The icosahedron-shaped NCLDVs have a roughly icosahedral outer capsid composed of hundreds of pseudo-hexameric capsomers in the icosahedral faces and one pentameric capsomer at each fivefold vertex. Each pentameric and pseudo-hexameric capsomer is composed of five copies of a penton protein and three copies of a major capsid protein (MCP), respectively. Immediately internal to the outer capsid shell is a layer of minor capsid proteins that stabilizes the outer capsid. PBCV-1 has an outer capsid with a diameter of ~190 nm, an inner bilayer lipid membrane that encloses a 331-kbp genome, and a minor capsid shell in-between the outer capsid shell and the inner membrane.

Here we have extended the fivefold averaged structure of PBCV-1 capsid to near-atomic resolution (~3.8 Å) and obtained an atomic model of the viral capsid by employing a symmetry relaxation procedure to distinguish the unique vertex with the other capsid vertices of PBCV-1, and the “block-based” reconstruction method. The atomic model contains 7135 polypeptide chains from 30 different kinds of proteins, with 15 kinds of the proteins previously unresolved. These previously unresolved proteins include five variants of the MCP that are involved in composing five types of pseudo-hexameric capsomers, one kind of penton protein variant that composes one type of pentameric capsomer, and nine kinds of minor capsid proteins. Type I, type II, type III and type IV capsomers are homotrimers of the MCP, MCPv1, MCPv3 and MCPv5, respectively, while type V and type VI capsomers are heterotrimers, with type V capsomer composed of two MCPv1 and one MCPv2 subunits, and type VI capsomer composed of two MCPv3 and one MCPv4 subunits. Type I capsomers are present in all the icosahedral asymmetric units, while type II and type V capsomers are only present in the unique vertex, with type II capsomers located at position a, b and type V capsomer located at position d, respectively. Each pentameric capsomer in the eleven common vertices of the viral capsid (hereafter “type I pentameric capsomer”) is composed of five penton protein (P1) monomers, whereas the pentameric capsomer in the unique vertex (hereafter “type II pentameric capsomer”) is composed of five monomers of the penton protein variant (P1v1). Compared with the type I pentameric capsomer, the type II pentameric capsomer has an ~7-nm-high “crown” structure formed by the DE insertion of its five P1v1 subunits. However, the association between the type II pentameric capsomer and its neighboring capsomers is reinforced by loop 179–197 of insertion domain I and the C-terminal bridging helix of P1v1. Below the type II pentameric capsomer is a lipid vesicle that has an ~7.3 × 104-Å3-large lumen, which is supported by minor capsid proteins P9, P15, P16, P17, and P18.

>[72x]MAGGLSQLVAYGAQDVYLTGNPQITFFKTVYRRYTNFAIESIQQTINGSVGFGNKVSTQISRNGDLITDIVVEFVLTKGGNGGTTYYPAEELLQDVELEIGGQRIDKHYNDWFRTYDALFRMNDDRYNYRRMTDWVNNELVGAQKRFYVPLIFFFNQTPGLALPLIALQYHEVKLYFTLASQVQGVNYNGSSAIAGAAQPTMSVWVDYIFLDTQERTRFAQLPHEYLIEQLQFTGSETATPSATTQASQNIRLNFNHPTKYLAWNFNNPTNYGQYTALANIPGACSGAGTAAATVTTPDYGNTGTYNEQLAVLDSAKIQLNGQDRFATRKGSYFNKVQPYQSIGGVTPAGVYLYSFALKPAGRQPSGTCNFSRIDNATLSLTYKTCSIDATSPAAVLGNTETVTANTATLLTALNIYAKNYNVLRIMSGMGGLAYAN;>MPGAISQLVSYGAQDVYLTGNPQITFFKAVYRRYTNFAMESIQQTFDGTTDFGKFPTVTISRNGDLAGPIWIEVNLPSLLGYNITPTPAEGNTSNIAAISTVFKDDYNNYWWTYNPGTTPQYSNLIAAFSNVDYKYYANAVTSTYPPTALSNVVYSWPYMITGNTGTRSTVAIPTANLRYVNGIGLALFNSIELELGGQRIDKHYSEWWDIWTELTETAEKIQGYNTMVGRYDPAVYNAGWNISQAQGGTYYVPLKFCYNRNPGLYMPLVALSYHQMKLNFNINNYLNCVKCNYPVTALTSKNGANPLSITNMKLYTDFVFLDAPERIRMSEIQHEYLVTQLQWQGSEPVTAPGDPNGSTNRKITLNFNHPVRELVFVYQAASNYDVDAVTGNNIFDYEIPANPTATPPYAGGGEVFTEVKLIINGSDRFSGRPGAYFRLVQPYEHHVRVPSKSVYVYSFALEDADSRQPNGSANFTRYDSVQLQLTLNENLASGRVQIYAPNFNILRIAAGMGGLAFAN[8x];> MDPTTRFRGSDVPVHNEDHMVFAKPSEIGLQGRQGFYTNTNVVTNTYNHVYTPPGGHTGGKFTQDIYTTDLLIAAKDEKADKIPLDKRMDGTFSEGTFVQLLSRGPQDVYLTYNPQISLFKRKYKRYTNFAIENFEERFSTVVKFGTRNICQLSKNGDLIGNMCFRVTLPNLGIPGGTWAPTMGYNIFSTIRMRIGDTIVQSHDRVWYDIDDKMFCDSTKIQGLDELIKRNVTLTTDQEWELIIPLKFFCCKRNTGKQQFLPILNMDTNINVYLEFNLLPLNSLVTLPTGSILPDIQSIDASVWVDYIFLDDTEKFRFAQDPCVYLIEQTASMDSLSYATTTSGQTYNKTDVYVDMKELNKPVKYVEIIAYEQGSTSFDYVDIIESATFYLNSDEQFKTRAGEYFSLVQPYQHFKRSDPTSNISTFSFALDAGSFQPNGYLNFAPYVRTRFAFKIQPQTTPHVIRLFAVCLNWVKFESGLVKLLFN;>MSGALNQLVAVGKQDAFITGDNLDNSVWRNVTKKVSNFAMESIENYINVNPGSTTSIVVGRFGDLVRKVTLEITMKKGSTTNPFYPSEQYVKYAHLSIGGQIVYRIDDFPTWTRVHEELFMDPDTRATNQRVNNFRPEDPVGAIRKFYLDIPLFFTDDASKALPLIALQYHEVKLDVLFASPGDIPGIDASYTPTVECYIDYVFLDTPEREWFARNTHMYVIEQLQHYNNVFSVAAVEQTKRLNLPFTMPTRYLIWLLKTGADGVYTTSGYPFENNDSYAAIKSAKLQFNGTDRFSERPGYYFTTVQPQDAFGRSPSAGIYVYSFGLDVTGMTSKGALNFSRMDNATLSITTKAATAATISDVYNQSTTLASAITDFTSIAIYAKSFNVLKIDYGMGGMLFAN[11x];>[4x]MVSGGVVQLISYGAQDVYISGGPKTIFKSYVKKVNNFAIDSVKIPINGMGNGNPSVLIPRNGDLIKSIRLEITLKKGTGQSFYPAEQLISYLALKIGGNIIQKIDDFSNFCRIRNELFMDPDERHTDYRVNNFSSSDVVGSVKYFFLDLPLFFSKDTSVALPLIALQYHDIELDFRFNDVSTIQGVDASYTPTIEMYIDYVYLEQQERIKLVEKPLFYNIEQCNFYRKDITFPALSSTFKLDIPFNNPSRFLVWYFNTDSFGIYNTSGLYFNSNDAAAPLESAVMLLNGTERFKSREGMYFNCVQPQQALGRSPSSGIYMYAFGEDVANATSKGALDMSRVNELSLQLTTKNATAANVYTVYNPQETLASSTSTYKGITLFSTNWNVLQVRSGLGAVMFDS;> MDDIETIEKYGRDETYIFLADSAKRDTAAYPTAAEYEVLFNAQFRNVTKFELLEVNIPRTEYLIDSSENTFAYALNQPTNINTWQQEIEGNIRIATITPGDYNLPQLIDEMNNVLQQTANTYGDSVILQVSPVTNPSEISNKIRITASGPFTLLGSTGTIGNTIGFGDPVNTSVASTTGYYSTVPGYSVNYPNGADYVFLSNQGNIGSEAVNEFVGPLPPGDNVSFTPIYTGQTPSQYFIAPSAGVPTTVSAYFVDQATAPPGGFVVNYSIIKVSDSSTIATGSLISTNDDLVPSVSSPSVVSANFIQGQQYYIQFTPGSSGSSAGNCTALWYSFPNLPPVSGAYAAINGTLVFPGQYFCTDVSAGAYGNELTSPGIVNITGARYIKIRCKELEQLIYRDRVGEPTTAGIGIVNLIGYGFERSRYDFSSIPVKAFHPIGKLQKLTFRLERPNGTLYDTNGVDNTMLCALTFKVVPNNAVDKTFDGPGKYPAAPGYSGDYIQLQQKRWGEEARATYPTHKSTYNRCRPRTT;> MCNTYYKRVKFNLFLYTNSIEMELLAVASIIGYGLFSSQQGRETRPDRNRYAEALGSGQGLDEDYDVKPTDMVRKYRKKAEKRWKKAQVPKESGIITPNMRPSEVMPYFTSGKSMNTNTDYKQRKMELFTGGVLDGHSVSGTYKHKVEAANMFGMTPQGRVTSDGTVGNAPGDTELLKARSVNSHQYNNVLPTEQLRVGPGLGVGPEVAATGGFHQFYRQLPLNINEYKLTQLPGRLVPGGTTTGGKGEIQQIASVNHNPDALVLNYDDRPPEATPNGAILASTQYGKQPRGYAGLRPYEKNYEGIAEADVSALQARYLDQTRGRPRTGDGDTEPIINPNGERDGTGSYVTENMCSMTLESQRGLVNRYITPPGVTGVVQQGGEMRPEFVPETTIREQYEDIYYTGPAGTTVTPTEPMNVVELQPESRHAKRAGQDRAYTPGAGRVNNFAPAAQGAYGLKDHPTYNALQHVVSEPIEQTFLPAAQGDDDRFGTKSNVNNPWGNPASLQIANNQLAANKFNRDVTNTVNLDYDAGQPMKQQNFQPKAWIPNNTDDMKMLPLWKRKQLQAQKNKQQRK;>MAMKTQRKENVLFQNVKPREIPLVDNPFSTYPYKHVITETQPTQAKNQAIWGLVQMGLSGEAAAMYGDVVVQKTTRACRKSEGGFKDVNTELWGTSPYLGRGDGEVYNMPASNQLLRGFESSLRGSRVRTQIDDKSFIPYTWQMIDVPLAAAKTSFIAGLDTRQQLAYGNP[3x];>MFSAFRDTASIGFSDTHQDEKTLRFLKKQISQFIKHLKEYYPNNELTKKLVMKYSDVQLLPYTKGATKDTYTSGLFDHTTGVIKIAPRDGLGNVRDEQSLNKSICHELAHGTRVKYPGESSHSDEWKDAWKTFLKIAADELGWKIEVPCSSVSFYGLTKDDCENCVWDQDPETCPKTAKLA[4x];> MDSRLSAAYAIRAARISMIPGGVDGLVINYAEGGEPAWVQYPLKKQKPLPNNLCYTPTLEDIARKREAVIAKYTKQPLETGTTFTHVLNASHLNEQYTRVKKSALPDKEFPIIETEKYPEPPILWETTIGAPSRLFDRSDGVKYVR;> MILVGIAVLILLAVFAILYYKQKEKFVVVGKFVEPIPSNPGQDFTLLPMDQTYTFADPVPDTATAFDVVLSRFTDKKAPADLLKGATFPEAAPYTDSEVENISKLALSRVKGPDAPVLSFISVEYAAKGVDNKKNTHYDIAFMVYDQVKNFSLKLVLVAVLDAKNKLWIKKFSSFNSFTPKDKGPKGVENIDETPLAEFIPDFVQFSRLYKDNANV;> METIGNFIQNMAFPTENPYKLSGDFGNSTLEPTVTAALRILHESPAPFNTEFFSRKNVDFIQKKLISETKRYTSFDIGPQNEDELIMMMAGIYVQDSTFDGNIKAGLRKLNTLVITECLKQILPGVRAYALYVRDASLPFSGGGEEAFKRPELATLKGSKVLSGFLPLDRNAS;> MKTETLYQDPVWFQDLSVIFKRPSEIIPTRDQSDSERINAMVRLVLYCSFAVALIRQNYLYAILGLAIIAIISLAYALGAKKTKSNEAYGNIRPYSVKRSKKSCSKSSANNPFSNATVGALLDNEARPPACSYDDNDMASTMRKNFNKGLFRNLDDVYEVENSQRQFYTMPVTTAAPDLTAFGQFLYGSKGKTCKEDPSACTPAFATRDG;>[12x]MDMHMIVKVVAILAVLFLVYKLWESMNKPNASPLKIQNPYEKYMNSAEGGEYDAEDDDIYYPETDAEDDDIYTGETDDMYDGEDDDIYVQEGDDIEDAEDEPYDDSADMEQDVPKVQQPMMPLLTPSSQLLPKPSPEAADFAQFAPKNLQAQNFLTATQWIGVNTQGSSLKNANYDLRADPIIPKADVGPWMMSSVDPNIYQKPLFG;>MFLYYKMNEVLNVNNGSSINVIKILKTPGPDIIRPGKTYKKKDVFTPKFFKNGNVMYTCNTFSLNVPVNNSIATIDFAEHVNGAVFKIEYNRVNFIAPSLYPISGLGTAVVFDLQKGEKASQRKITEFGNKDIRIADEISDIAADDHSVLITTKLMSESTPGELSRDVVLNGEIATGRINMNTGFVSDIIHTKKISIIDDGIVDYYVKINVPAKYSHGIVEVVSGTFLNDIMIHLVRNKNKWALMDSKMYIVNNTNGFVIAKNPDTAMGVSLLEWPRGAVVFPPYYNFKKFKNVNKWSISQQIASCVNTSVKIPGGEYSWKIRLFFGPIWQVQESINSVKTVPHGNDYMYLYKEEIVKYKYQRNTKRNFHEYDYDYKF[25x];>[8x]MSGYSNPLNDPIMIRTMIVYGNLSATYFTGNGAALTQQPIASNVPPTLRADAFGNVTSPANVISGNITTIDVISAGNINTRYVFGDGSTLSGISTGNSVVGVQKIDIIGNAVSSTISTGSLRTNVAFTNITANISNISYLSGNTVSNIINASNLIANIVNANVMSGDITLNRIVATDTRTINLFGNVSTNSFTAYGNVTANILTATTLTANSLQIESVSGNSVQKMIVGNLIGNVLTARTATFDTANIPTITSNVGIFTVANIRTITGDVRANVLNVSNIVTRSIGTDVVSNNIIATIGNVQSMIIGNLSANTLSVSNGTFQNFTTTVGLNVTTLSASVSNALVLSFTTGNSSSTTTTNLDAYGNTQFLRISTETSGINILNANSVSVGNLTIVGNVTSTSNNISGQVTSNSSQVQNINTNVIYSGNVFTSRFIAANANIRSLTASIGQVNSLTITSGNLTSLSFVNGNGNGVIATNANISNLNAVSMSGFAFDANVIIGDITANILSSGNLNANVFEANMLTSGNVVSTNGDTGTINANSIVLNVISGGDTRIDRLIANSVTTGDFYTTSTITAGVIDCAQGKISGNSSSNASLISNVISANTASFVNTSVGYGNLVNAVVIGNIIANVVTSGDANAVFLNSNLTTSGSIFGNISNSASIVAEYSNIRTMNVGNINSTTFNAEYLYVGNITVTGVSNTGYLICRNATFSLNSNIQTLITENVTTSNAGSNIFTNVITTGNAFSQNINTINANVLGITSVFSNVITNISNIRTLILLSNVSLGNLTATSANVTSNVSVGNLIGNIVASNAFFNTATIRNLAIFDVTGNILVAQSNASISNLTTERILLSDANIANLSTSNVSSNIAVVTGTCRIDAINSSNITFTNTATVSAAVVNVLGNLTVSNVINVQNLTANVGNIWQAVSNIQSMTTANIFTNTMTIINSFTYSNISSQRLIATNTLTANGVNLFSNIANLTVSGNANVGRWIAASAPATGALCFSSTESANLTTANLFAGNLNTWRAFVGNVIGNVMTTVAGDFGGIRVSVANIDVSGVANVENFTVNGNLFATNVITRDLSANLINFSGSLSNTSSISISGNSLFTSSANAANVGVSINMITQNLFGNRLSSENIQGNVLQASNIAVSQTVNVVGNISIGNLSVSRELFANSITISSGGTIVGNNTTRMITTPTSNSWSVGSLVGNANVSVQFTANTMVVQNIQPNTLVVNINQSTPTSNSGVRAIYIGYIVPVNFNATSSTTVSFSPALPTNCIYMPQLQYYSGGTVLQNNASFSTQIGLGVETITNTSCTIRMSTLDTLPIPSTSFFGLMVTAVQTV;>MSWFDPNWNPFFNRSIIVSGNLVVAGGVIEGNGGGLTNSAFSNPDTIRTDLTGNVTSNGTVRSSLIQTNSIVASGDAYANVWNGNAAFITGISANTTLVGNVRISISGNLTGNFAVSTTTVSNTMTANVLIGTTLTVNNLSATRANVQVLTGNVTGNVRLIANVVNVAAYTVGNLTTSSNVSTTNLNVTSNINGNVRSSTANVQGRLSATTPTTGSIISSSFIANSFTSSGNVQIGDFFGNVRASVGTFDMIASNVFSNVANIIEIRSDIISNIANVGNGTFVFVNASNITTTNITGNITSNVASFSNVDSIFGNVGNLRANTLTVTYANITGTLASGNVAVGNLISADNTSEFANITSFTTNGLVVNGNIIAAIGNGNVFLANVITANSLTLQSSSSTAASNVTTTRWIQSTTSTSNVMTIGNITSGNVISSNAAYFANVISNTITVMSAMTVSGNVSFGNVSFGNVSYGNITANVTTSTGNVSVDNLTSNVVNVVFCNASSVTANTLTSIALTGNTYVYSANTGVLTANVGNVFGTLTVGVANVTSMVSNALFANTAVVSNLSVSNLTVTISSDISNISITGNTSGNVFAANIATIGTLNTANVVANLVASNVMNAWVTSNIRTLITGNANVSTTTSNVITTGGFTITGNITSGLLTSNVIAGNITMYNTSNTTLFTSNTSNIANFFAGNMTAVNTIVSNLEIQGNSVVITQTTPFKVTSVLLANVLFANTIISNTFTTTANVVGNISTDIANIGIANVNFLNTTDFAVNTANIVNYTPTSNINVTGNLTLGNANIVNFYATSANIVGNITANNAVITFLTTPFYKGSGTVSAGFTSIISANALSNVIVFGNLSANIVVSNTLLSNSINVATVFSNVVNIGQVTSTGTTLVNSINFNISNVDVSGNVLVTRDVYTTNISVTTANIANVTFFSNVAIGNLISTRNLTAANLISSSDLFNSGPYTSSQNVTIDTLNFTAGNLGTVAARTTITTPTLFATDVNFTQDALVAGELITQNFYGNITSANIGSRITIGNANVTQTNITGNVVIPRTSNAAGFNSRLLISNNTTVTSNIVANSLISTGNIITNLLQTTGQVSFASLAVEYIDVANLAVRNVVTIGGNLTVSNVANLFSITANTVNMSTVTTNTLSANTITGTSNVLVAGNIIGNCFGNVLVNRGVVTGNVFADTITVPLNAVGVLTGNALIVPNTALHSVAITGSSAFTSNIRTLNTPNAFIWNTSVPSSGLLDARRLRFSQYITSNRIVEMRYFYITNALPQKYDSGGLNARYDLSFGTTLPTSQGQTWHHFLNTLYIGAQYNTNFSINCLIINATTTGLEVIIYNPFGIAASLSSSTPELYFYITSIATSTQ[4x];>MGGIMQLVSTGYQDVFLTGDPTRSLWKRIMARKTNFAIESIETVFDVLYGSTSFINIKKAGDLLKSCVLEITMKRTSTESFYPAEQFIKSLTLLIGDQEVEKIQDFPTWSRVHDELFNDTEMRSANYRMLNFRPDDPPGAIRTFYLDLPLFFTRYLSNSLPLVALQYHEVKLKIDFEPPYNIPGIDSTYMPQVRFYGDYVFLDKPERVYFAQTEHEYIIEQLQTFVTIPNMSNSVNTTMVDLPFTLPSRYIIWVYKTNLHGQYTTSNSTFVTNEGYAPLQSAVIKCNGTDRFSERPGGYFNMVQTTQALGQAPSCGIYMYSFGVNADKQDPEGTLNFSKLDMVTLSYTNKAATAADISQVFDLSTTLENGITKFKNITIFSKNFNVLRIVEGQGGILFSN[3x];>[3x]MGSYFVPPANYFFKDIFASNVGNIANVIFDNGNVIAAGGLGYLIGNGAFITGVTSTAIANIPAVVTADIRGNLIGNYANVNNIIASSGNISNVRFVSGGNVTASYYFGDGSQLTGITATANIPSIVTADIRGNIIGNYANVSNVSATFGNIANVLFNNGNVTAAGGNGFFIGNGSLLTGITATANIPSIVTADIRGNIIGNYANVSNVSATFGNIANVLFNNGNVTAAGGNGYFFGNGALLTGITATANIPSIVTADIRGNIIGNYANVSNVSATFGNIANVLFNNGNVTAAGGNGYFFGNGALLTGITATANIPSIVTADIRGNIIGNYANVSNVSATFGNIANVLFNNGNVTAAGGNGFFIGNGSLLSGITATANIPSIVTADIRGNIIGNYANVSNVTATFGNIANVLFNNGNVTAAGGNGYFFGNGSQLTGVTATLPSIVTADIRGNIIGNYANVSNVIATFGNIANVLFNNGNVTAADGNGYFFGNGSQLTGVTATLPSIVTADIRGNIIGNYANVSNVIATFGNIANVLFNNGNVTAAGGNGYFFGNGALLTGITATANIPSIVTADIRGNIIGNYANVSNVIATFGNIANVLFNNGNVTAADGNGYFFGNGSQLTGVTATLPSIVTADIRGNIIGNYANVSNVIATFGNIANVLFNNGNVTAAGGNGYFFGNGALLTGITATANIPSIVTADIRGNIIGNYANVSNVTATFGNIANVLFNNGNVTAAGGNGYFFGNGSQLTGVTATLPSIVTADIRGNIIGNYANVSNVIATFGNIANVLFNNGNVTAAGGNGYFFGNGALLTGITATANIPSIVTADIRGNIIGNYANVSNVTATFGNIGNVLFNNGNVTAAGGNGYFFGNGTFLNFSTITADIRGNIIGNYANVGNVIAGNVSTTLGNIGNVLFNNGNVTAAGGNGYFFGNGTSLTFSTIRADIRGNIIGNYANVANVIAGNVNSTFGNIAGVTFDAGNVSSPVDILVSGNVSVGSDGLFRGPTNQSNNALILRGIGGTNTVNLFSIGAPSGQMRFSVPASGVAFYNFLYGTNQVASLGPQGFYSLSYDSSVVVGQVVSNSTTYSGTIFKTEANRNSSTAFNHISCTGSNGNVFRVRGDGTTYGVGAFQTSGADYAEMMEWEDKNPTFEDRRGYPVVLSGNGKIRIASLSDDYNNIIGVVSSNPSMLADMAWDQWEGKYLKDKFGMRLSNTIYYLANISNENEFTRVGPMTTPPQGYFIKTSPEYILNPKYNPNVAYVERNDRPEWDPVGFVGKLRVRNGCLVHPSWKPLKVIDDYADVGNAAAQVTEYLIGVTPNYTLSKKVEDLEQTINVLKTQVQMLLGNI;> MGNGPPMERAVSSDDILTYYNTFIFFIYFNFTNENIYIIYTIYMKVQNTIVYIVLLLIVVVIIWNFTRKEGWSDYNAPNDFMKIYYSNIVEDKKLAEKYPFFGTGPFTGLRCRKPNNVGCNTTWVSGQLVELTPKLKEQIECKFGIQYVKT;> MHKITPFLIAAVVAVIVLAVWLFKKDNKKETWFSRDLNYGKANSKIWNATVAKGLKGIANENAEIRKMYPYLGYGDFTGAICKGPNNQGCTYYANYTR;> MWLFFFALAVIYMIYKRDVFKKIAVNLKMNGVSIPFVDKYSKQYPTYTKNALFHVTRFNNAYQKTFEYKNISIDTINNLFSIRDDVLYNISEIKLRLPNDLTQEKEINYMYEKTDQRLMEYITDVKSRFHINIYPGTMSSAFEARNYRASNDIVF;> MQGGLFGTIKLMIMLFSYFAAYQLGKMQERPQSQWPKAKAGQNKYMVGDWAAWKPIYMGVLGVAVLLTLLGPGGVGGGMGGMFGGGGGYGGYY;>MGAFTSFVLMLLFTGIILIATNELTYNRPREIQYRYLPRDLDSFIRTQEMPSAIFSSMWDVDTRRGGDGGPNPPGIRQSN[4x];>[2x]MTTITYDTDLLPPPELKVPSLDQALAPESVKNDDPFLDLSYFPVPKGFDNVGSLELNNLSTAEDVATLQNQLNKLAEEKHKRSTWKGLTFRIAVQDMWEALTGIPTDIYQNSGRVSLKELLTRDDRLRGLGLIFFLVAVVSIFFLAAG;>[3x]MASGWSDFRADPVIVNQDVVVFGNVFVDYLIGNASEMTGAADFVPGNVVNVNIIGNTVSTFVKSDVLMGDTITIDGNITATRLYGDASNMSGLPTLPPNANIDMVGNIVANTNTNKFVSVDTFTGDVTTNVATISNANVGTVTTNTTFFGNVITNVFNIGNLILTSSNVDTLNVTSLVASNVVSSQVDVQATIANSDLNVTRFDATSISAEIFVSSETLAVSNITNLIANIANIQGTTTVTGNLVGNIANVNTLTGNVTGNLFFTNLIIGNITANIFNTTTANVSNLITSNVSASNVSASNVTSTLFTIGNLNTNVATISNLFVTGTTIAGNTTFSSFSVSSLVANISGNNASIPTFTPNVLSTSNITIDGNAVVTGNAGFRTLNVTSLTANVLTTRGDVSNLYTDVINVNTNVFISSANILANNVITVQMNNISNVNITGNAEAFDVSANSVLMSTLSVGGILSLGNVNTNDISFGNIVTGNFFANFANVGNVQGNANVITMYSTTLTSNSAQIGNISGFSIVSNLGNAVSMFVGNLNTGTLVANNSTVGNITYISGNIGNANAQTVRVSGLLSASGVALTFNSITSNVAGNSLTVHGNLRTNSVTTEILTGNVGNLSILNTGNLFANSISVGQSFVISNFANAFIISSQTTNASVITANISGNIRVTNTLEANVVNSDSANIIIKNVSTSGNVSNTFTTGNLTVTNAVFRSGITGNNIEVVGNVNCDGNTTVTTLSYGNLITSVYNTRNIFGNITANTVNITNSNIGNVVTSNINANSLIITNLIPTVDITANVLRASQVNTGWFYGNATCNVLSMSNSVSINTLLSAEVFTSETINANANVSVATINSLGNTVAISRPSFLGNANIRLVISNVITIGNLTANTLVGDSFTATGIVNAINSNSQSDSIATNVTGNIIIRGNLILASSASAQSNASVFNPTNLISLNANSLSSLTATNVSANNVVISNTWQVSNLIVSNISAPNVTANSFQAISMTGRYYRPGISIERAGNLIVSNSLTSTANILQVLTSNTGQVNITNTMFGNISMSNIIVTGVVVTGNLTMGNVIANAVTTSVSTITGNATFGNLTVTDAVIIRGNITANNISTGSYIYGNGAFITGNLTSSGNANISIATRMFGTNSAINVAGTFTGVGNTNTTNATIANLTTNTLLSIGNLSTTGNFTVNSLSVGNLFANGSTIQLSNLANIQVSNLIYSGNVVVSNLSANTLSYVQNIGTSTQLQSGTMNVNNILSAGRFRLSISSTAPVFAGWTMGRVSLSGQSLRTNSGNPRTITFTTPLPAGYSYGIQLSVYSTVFGQTMALFNITVVSLTNTSVQFYIWNNPGGSGDSNTYIGYFAYAY> MFRISPSLAWRRTAAFYLRAGKLGQYEREAFEARRRLEESKNYPGPIRSATPGDTRFYAGSLESILQDNDRHYWRAVIDDPQVQYVIPLRIRFKLFTWVTTGWEQRLHIVQTMAPRDITIARLIELV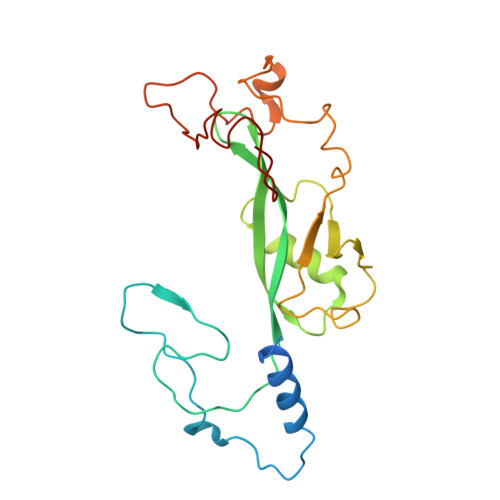TIENQSPYLCSSTFTLAVDGKELDPDKSLSDYGITEHSRIDAIEKLDHLLHKDSERPLDWTVDEMTTECLKRSPYKEMGMQPQPNLAPRYEARPKGYFGRNNYSGMKQES(2R)-2-AMINO-5-(3-METHYLPHENYL)-5,5-DIPHENYLPROPANOIC 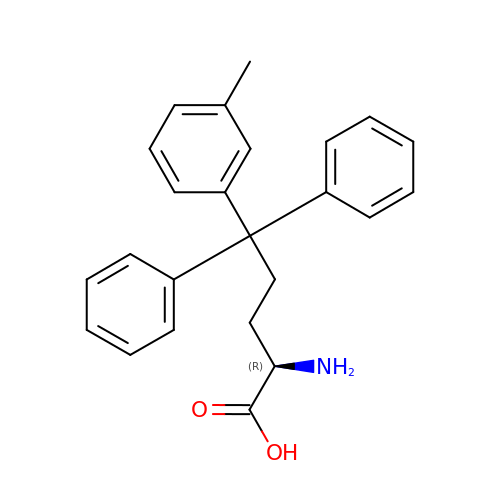ACID | C24 H25 N O2 | JXIGVUPYYZGRRZ-JOCHJYFZSA-N>[6x]SEGSHMGNRTFSYTLEDHTKQAFGIMNEL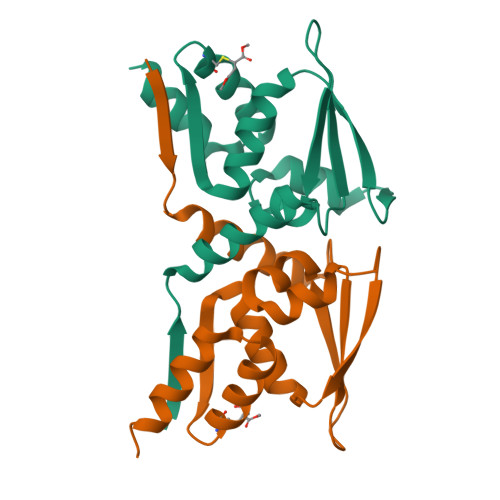RLSQQLCDVTLQVKYQDAPAAQFMAHKVVLASSSPVFKAMFTNGLREQGMEVVSIEGIHPKVMERLIEFAYTASISMGEKCVLHVMNGAVMYQIDSVVRACADFLVQQLD>[2x]MTATQITGVVLAAGRSNRLGTPKQLLPYRDTTVLGATLDVARQAGFDQLILTLGGAASAVRAAMALDGTDVVVVEDVE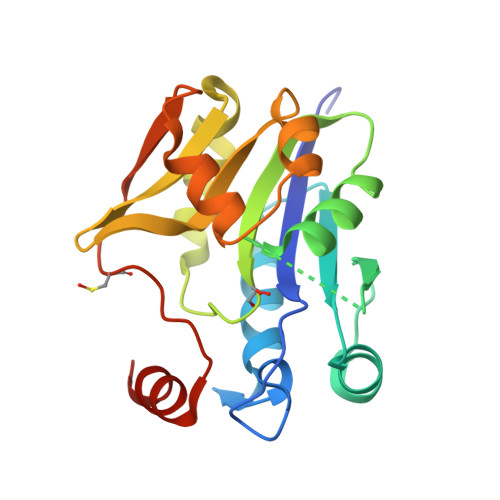RGCAASLRVALARVHPRATGIVLMLGDQPQVAPATLRRIIDVGPATEIMVCRYADGVGHPFWFSRTVFGELARLHGDKGVWKLVHSGRHPVRELAVDGCVPLDVDTWDDYRRLLESVPS> GSSLCLQRLQE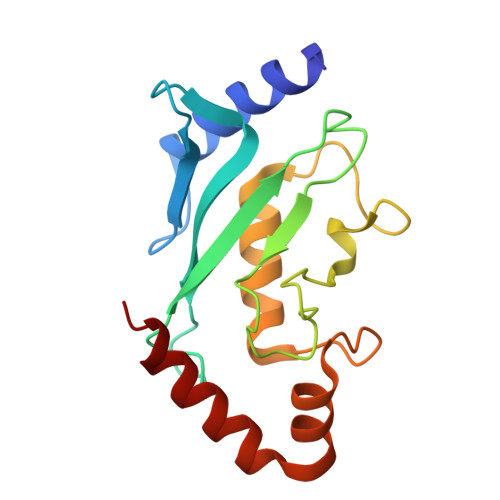ERKKWRKDHPFGFYAKPVKKADGSMDLQKWEAGIPGKEGTNWAGGVYPITVEYPNEYPSKPPKVKFPAGFYHPNVYPSGTICLSILNEDQDWRPAITLKQIVLGVQDLLDSPNPNSPAQEPAWRSFSRNKAEYDKKVLLQAKQYSK> GPVDNWRDNLVRQVQHSELELVANFADIPLRLSQILKLKPGDVLPIEKPDRIIAHVDGVPVLTSQYGTVNGQYALRVEHLINPILNSLNEEQPKNNPSDENTGALDDLWADALNEQKATTTKSAADAVFQQLGGGDVSGAMQDIDLIMDIPVKLTVELGRTRMTIKELLRLTQGSVVALDGLAGEPLDI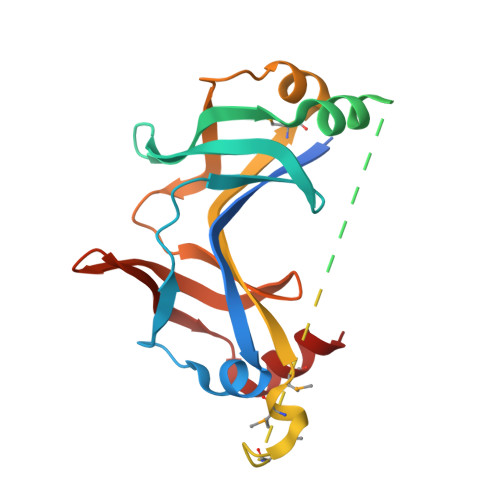LINGYLIAQGEVVVVADKYGVRITDIITPSERMRRLSR> SELYRQSLEIISRYLREQATGAKDTKP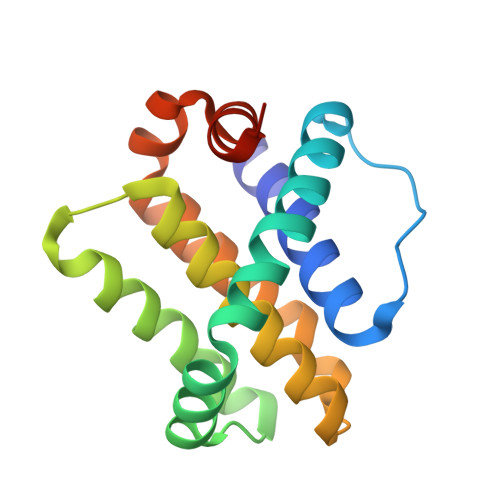MGRSGATSRKALETLRRVGDGVQRNHETAFQGMLRKLDIKNEDDVKSLSRVMIHVFSDGVTNWGRIVTLISFGAFVAKHLKTINQESCIEPLAESITDVLVRTKRDWLVKQRGWDGFVEFFHVEDLEGG5-CHLORO-N-(2-(4-(2-OXOPYRIDIN-1(2H)-YL)BENZAMIDO)ETHYL)THIOPHENE-2-CARBOXAMIDE | C19 H16 Cl N3 O3 S | 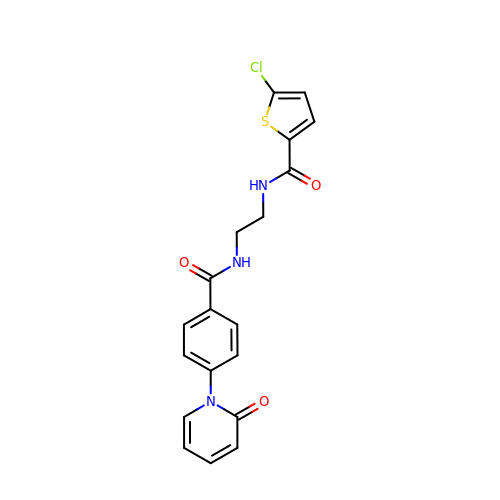UCKHUNHXYMAFQM-UHFFFAOYSA-N>KVTLYKTTATADSDKFKISQILTFNFIKDKSYDKDTLVLKATGNINSGFVKPNPNDYDFSKLYWGAKYNVSISSQSNDSVNVVDYAPKNQNEEFQVQNTLGYTFGGNTAFSETINYKQESYRTTLSRNTNYKNVGWGVEAHKIMNNGWGPYGRDSFHPTYGNELFLAGRQSSAYAGQNFIAQHQMPLLSRSNFNPEFLSVLSHRQDGAKKSKITVTYQREMDLYQIRWNGFYWAGANYKNFKTRTFKSTYEIDWENHKVKLLDTKETENNK[4x];>[4x]KIEDIGQGAEIIKRTQDITSKRLAITQNIQFDFVKDKKYNKDALVVKMQGFISSRTTYSDLKKYPYIKRMIWPFQYNISLKTKDSNVDLINYLPKNKIDSADVSQKLGYNIGSFNYSKTISYNQKNYVTEV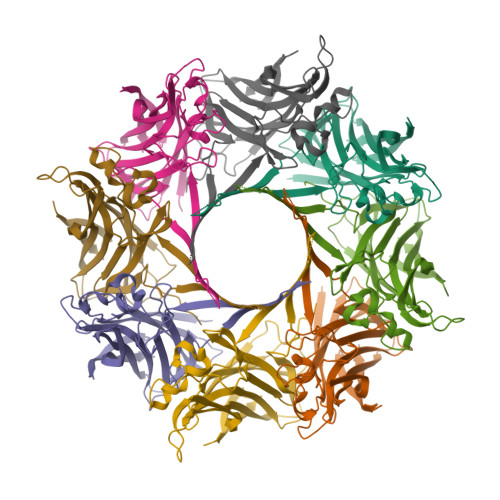ESQNSKGVKWGVKANSFVTPNGQVSAYDQYLFAQDPTGPAARDYFVPDNQLPPLIQSGFNPSFITTLSHERGKGDKSEFEITYGRNMDATYAYVTRHRLAVDRKHDAFKNRNVTVKYEVNWKTHEVKIKSITPK5'-O-[(R)-hydroxy{[(2E)-3-(4-oxocyclohexa-1,5-dien-1-yl)prop-2-enoyl]oxy}phosphoryl]adenosine 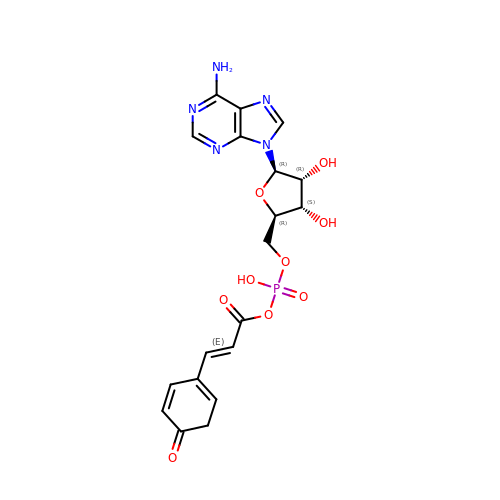| C19 H20 N5 O9 P | LAVNRUWSPLMSNH-PFQVGCJCSA-N>[3x]GSMGTPDPLTLRFTCLGDRNVIFFGPSGRQDGFTPLYDPSPSKRVATVDAGTYGLFIGGVGMNGEFADTIIEEARRNRIPLTATELSAESQEIQERLLHDAERQPGTLVEIDSGRFSRVFARSFAYVAIVPNTVWDE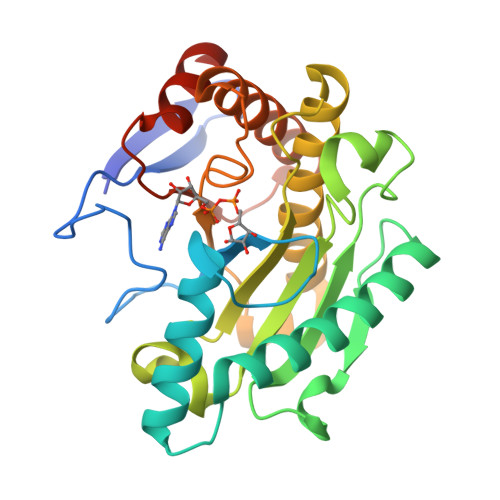SETGKNVGATFLHILKPEVTPHGNEMNDVMLYTVAPFGNASDSAYNMAYKATMLGIVGAVSEYNKTPWGEVKPVEAIRLPLLGAGHFRGRRGLHSIGRANAVAVEAAITRFDPRVELQFMYEPSDTALRGLMESERKYKFPQGD>[2x]GAAAAMSICPHIQQVFQNEKSKDGVLKTCNAARYILNHSVPKEKFLNTMKCGTCHEINSGATFMCLQCGFCGCWNHSHFLSHSKQIGHIFGINSNNGLLFCFKCEDYIGNIDLINDAILAKYWDDVCTKTMVPSMERRDGLSGLINMGNTCFMSSILQCLIHNPYFIRHSMSQIHSNNCKVRSPDKCFSCALDKIVHELYGALNTKQASSSSTSTNRQTGFIYLLTCAWKINQNLAGYSQQDAHEFWQFIINQIHQSYVLDLPNAKEVSRANNKQCECIVHTVFEGSLESSIVCP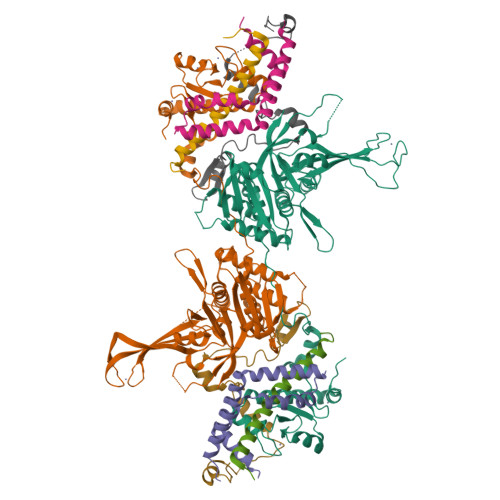GCQNNSKTTIDPFLDLSLDIKDKKKLYECLDSFHKKEQLKDFNYHCGECNSTQDAIKQLGIHKLPSVLVLQLKRFEHLLNGSNRKLDDFIEFPTYLNMKNYCSTKEKDKHSENGKVPDIIYELIGIVSHKGTVNEGHYIAFCKISGGQWFKFNDSMVSSISQEEVLKEQAYLLFYTIRQVN;>[2x]MTMDTAQLKSQIQQYLVESGNYELISNELKARLLQEGWVDKVKDLTKSEMNINESTNFTQILSTVEPKALEMVSDSTRETVLKQIREFLEEIVDTQ;>MTEETITIDSISNGILNNLLTTLIQDIVARETTQQQLLKTRYPDLRSYYFDPNGSLDINGLQKQQESSQYIH[2x];>MRSGDAEIKGIKPKVIEEYSLSQGSGPSNDSWKSLMSSAKDTPLQYDHMNRESLKKYFNPNAQLIEDPLDKPIQYRVCEKCGKPLALTAIVDHLEN[2x]> GIDPFTMSGDGSPPIHTRRQGFDPADELRAAGTLTKISIGSGADAETTWLAAGHAVVRQVLGDHKRFSTRRRFDRRDEIGGTGVFRPRELVGNLMDYDPPEHTRLRHLLTPGFTQRRMRRLAPRIEEIVTDRLDAMEQAGPPADLIELFADEVPGAVLCELIGVPRDDQAMFLQLCHRHLDASLSARKRAAAGEAFARYLVAMMARERKDPGDGFIGSIVAEHGDTITDEELRGVCVQLMLAGDDNVS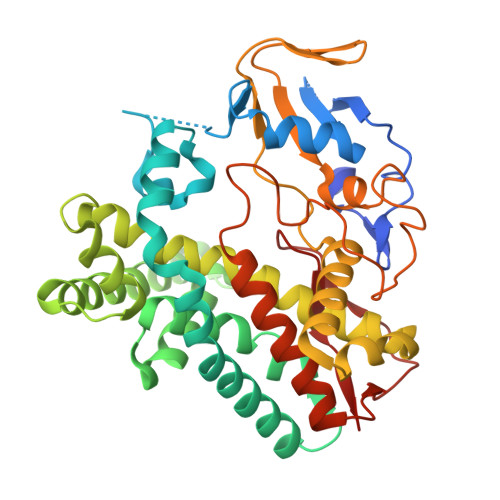GMIGLGVLALLRHPEQIAALRGDDQSADRAVDELIRYLTVPYAPTPRTAVEDVMVADQVIKEGETVLCSLPMANRDRALLPDADRLDVTRTPVPHVAFGHGIHHCLGAALTRLQLRIAYTALWRRFPALQLADPAQEIMFRTSTPAYGLTSLLVAW Peptide hormones, such as parathyroid hormone (PTH), neuropeptide Y (NPY), glucagon (GCG) and secretin (SCT), which adopt α-helical structures on binding their receptors, play key roles in human biology and are well-established biomarkers in clinical care and biomedical research. We set out to develop general methods for designing proteins that bind peptides in helical conformations. We show that by extending RFdiffusion8 to enable binder design to flexible targets, and to refining input structure models by successive noising and denoising (partial diffusion), picomolar-affinity binders can be generated to helical peptide targets by either refining designs generated with other methods, or completely de novo starting from random noise distributions without any subsequent experimental optimization. The deep learning methods largely converged on the overall solution to the helical peptide-binding design problem—groove-shaped scaffolds with helices lining the binding site—that the human designers chose in the initial Rosetta parametric approaches.

As a first experimental test of partial diffusion, we started from our parametrically designed Inpainted binders to GCG (with 231 nM Kd) and NPY (with 3.5 µM affinity). Following partial noising and denoising, we identified diverse designs that in silico had substantially improved computational metrics compared to the starting design. The highest-affinity designs were expressed in E. coli and then purified, and their binding affinities were determined using FP to be 5.6 nM to NPY (top) and below the limit of detection in the picomolar range to GCG (bottom). To gain insight into the structural rearrangements generated by partial diffusion that contribute to the affinity increases, we solved the structures of the original Inpainted GCG binder and the partially diffused higher-affinity GCG binder. Both designs were very close to their design models. Subtle structural changes in the protein backbone between the original Inpainted design model and the partially diffused model are nearly perfectly recapitulated in the corresponding crystal structures. Alignment of the two crystal structures on the structurally conserved C-terminal residues (16–29) of GCG showed that in the partially diffused GCG binder a 2.7-Å shift towards the target in the binder backbone enables an isoleucine to fit into a pocket previously occupied by a phenylalanine side chain at position 13 (left inset).

> MSGSMEKLAEIMQEIIEAYQEVKDAFFKFIKAVHEGAPEEELKKYLEKMKEALEKMKELLERLEKEAKKVIEENKDKKLELKVLLMLRLAYLLLKVSIELTKIAAEKLGDKELVEELEKESKEVEKKIKELEERIKKLLEEVDDEELKEAYKEVEEMEKEAEKFLEKMRKVGSG;> HSQGTFTSDYSKYLDSRRAQDFVQWLMNT>[2x]GPLGSMASFKLATDLPEWKKLEETYKSVGEKFSVRDAFAKDPKRFEEFSWIYKNYDDSKILFDFSKNLVNKEILDQLVTLAKEAGVEKLRDAMFAGDHINTTEDRAVYHVALRNRALRKMPVDGKDTAQEVDDVLKHMKEFSDSIRDGSWTGYTGKSITDVVNIGIGGSDLGPVMVTEALKAYSKPGLNVHFISNIDGTHTAETLKNLNPETTLFLIASKTFTTAETITNATS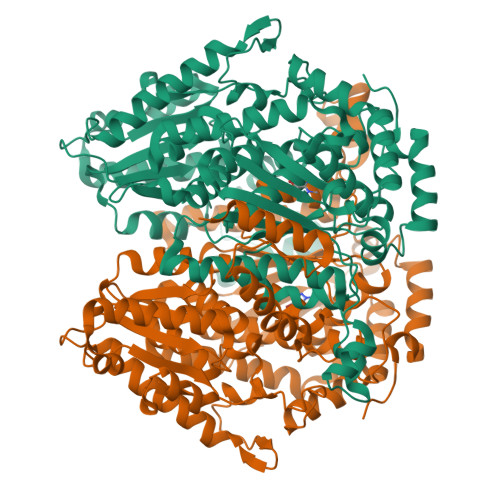AKNWFLATAKDSKHIAKHFAALSTNEKEVVAFGIDAKNMFGFESWVGGRYSVWSAIGLSVAIYIGFENFNDFLKGAEAMDQHFLTTPLENNIPVIGGLLSVWYNNFFGAQTHLVVPFDQYLHRFPAYLQQLSMESNGKSVTRANVFTNYQTGTILFGEPATNAQHSFFQLVHQGTKLIPADFILAAQSHNPIEKNLHQRMLASNFFAQSEALMVGKDEAKVKAEGATGGLVPHKEFSGNRPTTSILAQKITPATLGSLIAYYEHLTFTEGAIWNINSFDQWGVELGKVLAKVIGKELDDKKAVATHDASTNGLINQFKEWEE> GPMEDLIPLVNRLQDAFSAIGQNADLDLPQIAVVGGQSAGKSSVLENFVGRDFLPRGSGIVTRRPLVLQLVNATTEYAEFLHCKGKKFTDFEEVRLEI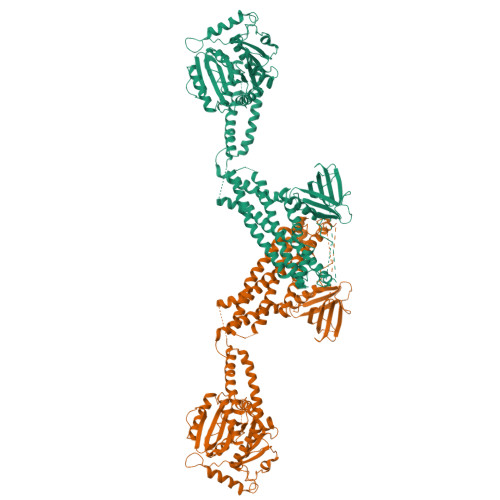EAETDRVTGTNKGISPVPINLRVYSPHVLNLTLVDLPGMTKVPVGDQPPDIEFQIRDMLMQFVTKENCLILAVSPANSDLANSDALKVAKEVDPQGQRTIGVITKLDLMDEGTDARDVLENKLLPLRRGYIGVVNRSQKDIDGKKDITAALAAERKFFLSHPSYRHLADRMGTPYLQKVLNQQLTNHIRDTLPGLRNKLQSQLLSIEKEVEEYKNFRPDDPARKTKALLQMVQQFAVDFEKRIEGSGDQIDTYELSGGARINRIFHERFPFELVKMEFDEKELRREISYAIKNAAAAATGLFTPDMAFETIVKKQVKKIREPCLKCVDMVISELISTVRQCTKKLQQYPRLREEMERIVTTHIREREGRTKEQVMLLIDIELAYMNTNHEDFIGFANAQQRSNQMNKKKTSGNQDEILVIRKGWLTINNIGIMKGGSKEYWFVLTAENLSWYKDDEEKEKEYMLSVDNLKLRDVEKGFMSSKHIFALFNTEQRNVYKDYRQLELACETQEEVDSWKASFLRAGVYPERVGDKEKASETEENGSDSFMHSMDPQLERQVETIRNLVDSYMAIVNKTVRDLMPKTIMHLMINNTKEFIFSELLANLYSCGDQNTLMEESAEQAQRRDEMLRMYHALKEALSIIGDIN Upon termination, the replisome is disassembled in two steps: first, CMG is ubiquitylated on its Mcm7 subunit by a cullin-RING E3 ubiquitin ligase (SCFDia2 in budding yeast, CUL2LRR1 in metazoa); second, ubiquitylated Mcm7 is unfolded by the Cdc48 ATPase (also known as p97 in higher eukaryotes), leading to disassembly of the replisome. Despite being driven by evolutionarily diverse E3 ubiquitin ligases in different eukaryotes (SCFDia2 in budding yeast, CUL2LRR1 in metazoa), replisome disassembly is governed by a common regulatory principle, in which ubiquitylation of CMG is suppressed before replication termination, to prevent replication fork collapse. Our structures show that the leucine-rich repeat domains of Dia2 and LRR1 are structurally distinct, but bind to a common site on CMG, including the MCM3 and MCM5 zinc-finger domains. The LRR–MCM interaction is essential for replisome disassembly and, crucially, is occluded by the excluded DNA strand at replication forks, establishing the structural basis for the suppression of CMG ubiquitylation before termination.

Nonetheless, we identified a subset of particles, which was subsequently subclassified into two conformations (conformations I and II), that had unambiguously translocated onto dsDNA, representative of bona fide termination intermediates produced after fork convergence. While the configuration of the MCM C-tier differed between conformations I and II, in both cases the incoming dsDNA was bent by approximately 46° between the MCM N-tier and C-tier, necessitating distortion of the DNA duplex within the N-tier. Having identified particles that had translocated onto dsDNA, we were able to build an atomic model of a terminated replisome. We observed an additional, large region of density at the N-tier face of CMG beside Mcm3 and Mcm7, which closely approaches Csm3 and the dsDNA ahead of CMG, before extending away from the core of the complex, forming an elongated arm characteristic of the cullin subunit (Cdc53) of SCFDia2. Density corresponding to the E3 ligase substrate-recognition module (Skp1–Dia2) is adjacent to the N-tier face of CMG. However, clearsecondary structure and side chain density enabled us to build a de novo atomic model for the remainder of Dia2, encompassing the F-box (residues 211–247), 15 tandem leucine-rich repeats (LRRs) (248–716) and a C-terminal tail (717–732), which folds back onto the concave surface of the horseshoe-shaped LRRs. The C-terminal end of the LRR domain forms an extensive interface with the N-tier of the Mcm3, Mcm5 and Mcm7 subunits of CMG (see text below for a detailed description), demonstrating that Dia2 binds directly to CMG bound around dsDNA, equivalent to the situation after convergence of two replication forks. The extensive interface between Dia2LRR and MCM is predominantly formed by the Mcm3 N-tier (helices α1 and α5 and the zinc-finger (ZnF) domain), which forms a cradle for the C terminus of Dia2LRR.

> MSDNRRRRREEDDSDSENELPPSSPQQHFRGGMNPVSSPIGSPDMINPEGDDNEVDDVPDIDEVEEQMNEVDLMDDNMYEDYAADHNRDRYDPDQVDDREQQELSLSERRRIDAQLNERDRLLRNVAYIDDEDEEQEGAAQLDEMGLPVQRRRRRRQYEDLENSDDDLLSDMDIDPLREELTLESLSNVKANSYSEWITQPNVSRTIARELKSFLLEYTDETGRSVYGARIRTLGEMNSESLEVNYRHLAESKAILALFLAKCPEEMLKIFDLVAMEATELHYPDYARIHSEIHVRISDFPTIYSLRELRESNLSSLVRVTGVVTRRTGVFPQLKYVKFNCLKCGSILGPFFQDSNEEIRISFCTNCKSKGPFRVNGEKTVYRNYQRVTLQEAPGTVPPGRLPRHREVILLADLVDVSKPGEEVEVTGIYKNNYDGNLNAKNGFPVFATIIEANSIKRREGNTANEGEEGLDVFSWTEEEEREFRKISRDRGIIDKIISSMAPSIYGHRDIKTAVACSLFGGVPKNVNGKHSIRGDINVLLLGDPGTAKSQILKYVEKTAHRAVFATGQGASAVGLTASVRKDPITKEWTLEGGALVLADKGVCLIDEFDKMNDQDRTSIHEAMEQQSISISKAGIVTTLQARCSIIAAANPNGGRYNSTLPLAQNVSLTEPILSRFDILCVVRDLVDEEADERLATFVVDSHVRSHPENDEDREGEELKNNGESAIEQGEDEINEQLNARQRRLQRQRKKEEEISPIPQELLMKYIHYARTKIYPKLHQMDMDKVSRVYADLRRESISTGSFPITVRHLESILRIAESFAKMRLSEFVSSYDLDRAIKVVVDSFVDAQKVSVRRQLRRSFAIYTLGH;> MKRRWKKNFIAVSAANRFKKISSSGALENLYFQGEAPVMEGSTGFDGDATTFFAPDAVFGDRVRRFQEFLDTFTSYRDSVRSIQVYNSNNAANYNDDQDDADERDLLGDDDGDDLEKEKKAASSTSLNILPHRIIISLDDLREFDRSFWSGILVEPAYFIPPAEKALTDLADSMDDVPHPNASAVSSRHPWKLSFKGSFGAHALSPRTLTAQHLNKLVSVEGIVTKTSLVRPKLIRSVHYAAKTGRFHYRDYTDATTTLTTRIPTPAIYPTEDTEGNKLTTEYGYSTFIDHQRITVQEMPEMAPAGQLPRSIDVILDDDLVDKTKPGDRVNVVGVFKSLGAGGMNQSNSNTLIGFKTLILGNTVYPLHARSTGVAARQMLTDFDIRNINKLSKKKDIFDILSQSLAPSIYGHDHIKKAILLMLMGGVEKNLENGSHLRGDINILMVGDPSTAKSQLLRFVLNTASLAIATTGRGSSGVGLTAAVTTDRETGERRLEAGAMVLADRGVVCIDEFDKMTDVDRVAIHEVMEQQTVTIAKAGIHTTLNARCSVIAAANPVFGQYDVNRDPHQNIALPDSLLSRFDLLFVVTDDINEIRDRSISEHVLRTHRYLPPGYLEGEPVRERLNLSLAVGEDADINPEEHSNSGAGVENEGEDDEDHVFEKFNPLLQAGAKLAKNKGNYNGTEIPKLVTIPFLRKYVQYAKERVIPQLTQEAINVIVKNYTDLRNDDNTKKSPITARTLETLIRLATAHAKVRLSKTVNKVDAKVAANLLRFALLGEDIGNDIDEEESEYEEALSKRSPQKSPKKRQRVRQPASNSGSPIKSTPRRSTASSVNATPSSARRILRFQDDEQNAGEDDNDIMSPLPADEEAELQRRLQLGLRVSPRRREHLHAPEEGSSGPLTEVGTPRLPNVSSAGQDDEQQQSVISFDNVEPGTISTGRLSLISGIIARLMQTEIFEEESYPVASLFERINEELPEEEKFSAQEYLAGLKIMSDRNNLMVADDKVWRV;> MSQQSSSPTKEDNNSSSPVVPNPDSVPPQLSSPALFYSSSSSQGDIYGRNNSQNLSQGEGNIRAAIGSSPLNFPSSSQRQNSDVFQSQGRQGRIRSSASASGRSRYHSDLRSDRALPTSSSSLGRNGQNRVHMRRNDIHTSDLSSPRRIVDFDTRSGVNTLDTSSSSAPPSEASEPLRIIWGTNVSIQECTTNFRNFLMSFKYKFRKILDEREEFINNTTDEELYYIKQLNEMRELGTSNLNLDARNLLAYKQTEDLYHQLLNYPQEVISIMDQTIKDCMVSLIVDNNLDYDLDEIETKFYKVRPYNVGSCKGMRELNPNDIDKLINLKGLVLRSTPVIPDMKVAFFKCNVCDHTMAVEIDRGVIQEPARCERIDCNEPNSMSLIHNRCSFADKQVIKLQETPDFVPDGQTPHSISLCVYDELVDSCRAGDRIEVTGTFRSIPIRANSRQRVLKSLYKTYVDVVHVKKVSDKRLDVDTSTIEQELMQNKVDHNEVEEVRQITDQDLAKIREVAAREDLYSLLARSIAPSIYELEDVKKGILLQLFGGTNKTFTKGGRYRGDINILLCGDPSTSKSQILQYVHKITPRGVYTSGKGSSAVGLTAYITRDVDTKQLVLESGALVLSDGGVCCIDEFDKMSDSTRSVLHEVMEQQTISIAKAGIITTLNARSSILASANPIGSRYNPNLPVTENIDLPPPLLSRFDLVYLVLDKVDEKNDRELAKHLTNLYLEDKPEHISQDDVLPVEFLTMYISYAKEHIHPIITEAAKTELVRAYVGMRKMGDDSRSDEKRITATTRQLESMIRLAEAHAKMKLKNVVELEDVQEAVRLIRSAIKDYATDPKTGKIDMNLVQTGKSVIQRKLQEDLSREIMNVLKDQASDSMSFNELIKQINEHSQDRVESSDIQEALSRLQQEDKVIVLGEGVRRSVRLNNRV;> MSFDRPEIYSAPVLQGESPNDDDNTEIIKSFKNFILEFRLDSQFIYRDQLRNNILVKNYSLTVNMEHLIGYNEDIYKKLSDEPSDIIPLFETAITQVAKRISILSRAQSANNNDKDPENTSMDTDSLLLNSLPTFQLILNSNANQIPLRDLDSEHVSKIVRLSGIIISTSVLSSRATYLSIMCRNCRHTTSITINNFNSITGNTVSLPRSCLSTIESESSMANESNIGDESTKKNCGPDPYIIIHESSKFIDQQFLKLQEIPELVPVGEMPRNLTMTCDRYLTNKVIPGTRVTIVGIYSIYNSKNGAGSGRSGGGNGGSGVAIRTPYIKILGIQSDVETSSIWNSVTMFTEEEEEEFLQLSRNPKLYEILTNSIAPSIFGNEDIKKAIVCLLMGGSKKILPDGMRLRGDINVLLLGDPGTAKSQLLKFVEKVSPIAVYTSGKGSSAAGLTASVQRDPMTREFYLEGGAMVLADGGVVCIDEFDKMRDEDRVAIHEAMEQQTISIAKAGITTVLNSRTSVLAAANPIYGRYDDLKSPGDNIDFQTTILSRFDMIFIVKDDHNEERDISIANHVINIHTGNANAMQNQQEENGSEISIEKMKRYITYCRLKCAPRLSPQAAEKLSSNFVTIRKQLLINELESTERSSIPITIRQLEAIIRITESLAKLELSPIAQERHVDEAIRLFQASTMDAASQDPIGGLNQASGTSLSEIRRFEQELKRRLPIGWSTSYQTLRREFVDTHRFSQLALDKALYALEKHETIQLRHQGQNIYRSGV;> MSSPFPADTPSSNRPSNSSPPPSSIGAGFGSSSGLDSQIGSRLHFPSSSQPHVSNSQTGPFVNDSTQFSSQRLQTDGSATNDMEGNEPARSFKSRALNHVKKVDDVTGEKVREAFEQFLEDFSVQSTDTGEVEKVYRAQIEFMKIYDLNTIYIDYQHLSMRENGALAMAISEQYYRFLPFLQKGLRRVVRKYAPELLNTSDSLKRSEGDEGQADEDEQQDDDMNGSSLPRDSGSSAAPGNGTSAMATRSITTSTSPEQTERVFQISFFNLPTVHRIRDIRSEKIGSLLSISGTVTRTSEVRPELYKASFTCDMCRAIVDNVEQSFKYTEPTFCPNPSCENRAFWTLNVTRSRFLDWQKVRIQENANEIPTGSMPRTLDVILRGDSVERAKPGDRCKFTGVEIVVPDVTQLGLPGVKPSSTLDTRGISKTTEGLNSGVTGLRSLGVRDLTYKISFLACHVISIGSNIGASSPDANSNNRETELQMAANLQANNVYQDNERDQEVFLNSLSSDEINELKEMVKDEHIYDKLVRSIAPAVFGHEAVKKGILLQMLGGVHKSTVEGIKLRGDINICVVGDPSTSKSQFLKYVVGFAPRSVYTSGKASSAAGLTAAVVRDEEGGDYTIEAGALMLADNGICCIDEFDKMDISDQVAIHEAMEQQTISIAKAGIHATLNARTSILAAANPVGGRYNRKLSLRGNLNMTAPIMSRFDLFFVILDDCNEKIDTELASHIVDLHMKRDEAIEPPFSAEQLRRYIKYARTFKPILTKEARSYLVEKYKELRKDDAQGFSRSSYRITVRQLESMIRLSEAIARANCVDEITPSFIAEAYDLLRQSIIRVDVDDVEMDEEFDNIESQSHAASGNNDDNDDGTGSGVITSEPPADIEEGQSEATARPGTSEKKKTTVTYDKYVSMMNMIVRKIAEVDREGAEELTAVDIVDWYLLQKENDLGSLAEYWEERRLAFKVIKRLVKDRILMEIHGTRHNLRDLENEENENNKTVYVIHPNCEVLDQLEPQDSS;> MSAALPSIQLPVDYNNLFNEITDFLVTFKQDTLSSDATRNENEDENLDAENIEQHLLEKGPKYMAMLQKVANRELNSVIIDLDDILQYQNEKFLQGTQADDLVSAIQQNANHFTELFCRAIDNNMPLPTKEIDYKDDVLDVILNQRRLRNERMLSDRTNEIRSENLMDTTMDPPSSMNDALREVVEDETELFPPNLTRRYFLYFKPLSQNCARRYRKKAISSKPLSVRQIKGDFLGQLITVRGIITRVSDVKPAVEVIAYTCDQCGYEVFQEVNSRTFTPLSECTSEECSQNQTKGQLFMSTRASKFSAFQECKIQELSQQVPVGHIPRSLNIHVNGTLVRSLSPGDIVDVTGIFLPAPYTGFKALKAGLLTETYLEAQFVRQHKKKFASFSLTSDVEERVMELITSGDVYNRLAKSIAPEIYGNLDVKKALLLLLVGGVDKRVGDGMKIRGDINVCLMGDPGVAKSQLLKAICKISPRGVYTTGKGSSGVGLTAAVMKDPVTDEMILEGGALVLADNGICCIDEFDKMDESDRTAIHEVMEQQTISISKAGINTTLNARTSILAAANPLYGRYNPRLSPLDNINLPAALLSRFDILFLMLDIPSRDDDEKLAEHVTYVHMHNKQPDLDFTPVEPSKMREYIAYAKTKRPVMSEAVNDYVVQAYIRLRQDSKREMDSKFSFGQATPRTLLGIIRLSQALAKLRLADMVDIDDVEEALRLVRVSKESLYQETNKSKEDESPTTKIFTIIKKMLQETGKNTLSYENIVKTVRLRGFTMLQLSNCIQEYSYLNVWHLINEGNTLKFVDDGTMDTDQEDSLVSTPKLAPQTTASANVSAQDSDIDLQDA;> MYGDLGNKLVLEAKRTKQLYARSNQDVNLPMYHEDIIRNILKEVSNLRKNTEYLKEQQQLGMLDDKVAKCQYFVTLLCMERNKRCLLAYQRLRTDILDSMAWNNNGLDLMSSITFSQQDTNNLSHQEQEYLKEYCDLITDLKSGDLVDIDLSGSLVPPSDVFIDVRVLKDAGEIQTEYGVFNLIKDSQFFVRQSDVERLIQQGYLQKI;> MSLPAHLQQTFSPEEIQFIVENEPIKIFPRITTRQKIRGDDRGTGNHTRWQLITTDDKALNNMVAMRSTEVVLWIALLLKQQSKCSIVAPQWLTTKELDRKIQYEKTHPDRFSELPWNWLVLARILFNKAKDDFHDPIHELRGKIQDLREIRQIKVLKGLKYLNESHLQLDNLSLLEINELRPFITEIMDKLREIHTASLTAGTENDEEEFNI;> MGYYDIDDVLADGTEFPCKFQYDIPGLGYLENNPGRPITKNTKLNLPLWLARILAIVGGDEALVDEEPVPFVELLPPDMFSTKVMNAIKTDPVALDLHSINSHFFSLAIKWIMLFSEKELANVVSELLLQRAQELNHHASSLSIDLNADSTGKNSANTNIATSTFLLKLEEMEKEIYKKSHESYKDTKRWMFKK;> MDINIDDILAELDKETTAVDSTKITQGSSSTTHRDANTIVGSSLDLNDKTQIYVSPQQDFSDLMKSWKNERCSPELLPYPHQLMKRLLNRISMQSQLIENISMGFLDMQNASNANPPMPNESKLPLLCMETELERLKFVIRSYIRCRLSKIDKFSLYLRQLNEDENSLISLTDLLSKDEIKYHDTHSLIWLKLVNDSILKYMPEELQAINDTEGSVNMIDEPDWNKFVFIHVNGPPDGKWNEDPLLQENEFGKPCYTVTIPDLKEEVELTIGSIYVMRYEVIRDLLRDDKVALI;> MYYGISQFSEAYNKILRNSSSHSSCQLVIFVSCLNIDALCATKMLSLLFKKQLVQSQIVPIFGYSELRRHYSQLDDNINSLLLVGFGGVIDLEAFLEIDPQEYVIDTDEKSGEQSFRRDIYVLDAHRPWNLDNIFGSQIIQCFDDGTVDDTLGEQKEAYYKLLELDEESGDDELSGDENDNNGGDDEATDADEVTDEDYKDDDGDYKDDDETISNKRGNSSIGPNDLSKRKQRKKQIHEYEGVLEEYYSQGTTVVNSISAQIYSLLSAIGETNLSNLWLNILGTTSLDIAYAQVYNRLYPLLQDEVKRLTPSSRNSVKTPDTLTLNIQPDYYLFLLRHSSLYDSFYYSNYVNAKLSLWNENGKKRLHKMFARMGIPLSTAQETWLYMDHSIKRELGIIFDKNLDRYGLQDIIRDGFVRTLGYRGSISASEFVEALTALLEVGNSTDKDSVKINNDNNDDTDGEEEEDNSAQKLTNLRKRWVSNFWLSWDALDDRKVELLNRGIQLAQDLQRAIFNTGVAILEKKLIKHLRIYRLCVLQDGPDLDLYRNPLTLLRLGNWLIECCAESEDKQLLPMVLASIDENTDTYLVAGLTPRYPRGLDTIHTKKPILNNFSMAFQQITAETDAKVRIDNFESSIIEIRREDLSPFLEKLTLSGLL;>[3x]MKRRWKKNFIAVSAANRFKKISSSGALENLYFQGEMVSVIDKLVFDFGGKTLVSLAPDNNTLCVANKNGLTKILKTNNPEEEPETLDSSKLVSSIKCYSNSHFLMTTMQGDALRYNIDSSQEELLARFALPLRDCCVIHSGKMAVFGGDDLELILLELDDETHKKHAIKIDEQVSQISYNSQMNILAVSMINGKVQIFSLTSTIPNKVHELNDYIVANSYDDTHRDKILSNMMDDIDKDNDNDLSETADPDENNVADPEFCAANRICTRVAWHPKGLHFALPCADDTVKIFSIKGYSLQKTLSTNLSSTKAHFIDLQFDPLRGTYIAAVDLNNKLTVWNWETSEIHYTREFKRKITNIAWKIQADSKTLDLVLGTWSGSIAIVQNLAESVVSNIPDQSVAESSTKHGLFVDSESDLENLEGNDDINKSDKLFSDITQEANAEDVFTQTHDGPSGLSEKRKYNFEDEEDFIDDDDGAGYISGKKPHNEHSYSRVHKTHSFPISLANTGKFRYMPFSPAGTPFGFTDRRYLTMNEVGYVSTVKNSEQYSITVSFFDVGRFREYHFEDLFGYDLCFLNEKGTLFGQSKTGQIQYRPHDSIHSNWTKIIPLQAGERITSVAATPVRVIVGTSLGYFRSFNQFGVPFAVEKTSPIVALTAQNYRVFSVHYSQFHGLSYSLSELGTSSKRYYKRECPLPMSLPNINSDMKKDANLDYYNFNPMGIKSLFFSSYGDPCIFGSDNTLLLLSKWRSPEESKWLPILDSNMEIWKMSGGKETTDIHVWPLALAYDTLNCILVKGKHIWPEFPLPLPSEMEIRMPVFVKSKLLEENKAILNKKNEIGADTEAEEGEEDKEIQIPVSMAAEEEYLRSKVLSELLTDTLENDGEMYGNENEVLAALNGAYDKALLRLFASACSDQNVEKALSLAHELKQDRALTAAVKISERAELPSLVKKINNIREARYEQQLK;> MVTSNVVLVSGEGERFTVDKKIAERSLLLKNYLNDMHDSNLQNNSDSESDSDSETNHKSKDNNNGDDDDEDDDEIVMPVPNVRSSVLQKVIEWAEHHRDSNFPDEDDDDSRKSAPVDSWDREFLKVDQEMLYEIILAANYLNIKPLLDAGCKVVAEMIRGRSPEEIRRTFNIVNDFTPEEEAAIRRENEWAEDR;> GAGMSSPGNSGVAIDSTVLKAIELGTRLFKSGEYLQAKRIFTNALRVCDSYSQEQIMRIRNAYQLDTARPDNKRLYHPRYIKILDNICACYEKLNDLKSCLDVSQRLLKLEPGNIKCYIRCTRTLIKLKDWKRAYKTCSRGLQLCNNDSNHLRQQKQFIKNNMVQKQDGKRSYIDPLEETKIAKKKKNNNVLESLPKKKIKGSTKKTDLVGNLPIEILPIIFQRFTTKELVTLSLVCNKWRDKILYHLDCFQEFNLAPINFKNFVKFMDFLQQNFTRTYRKYILSQVKVSSRITSEELRITQLLFSKMPKCINIERLILSMPTLTTTQIFKLMVRGGTDFFTRLLELSLMITYRPDKQHELEILQTCPLLKKIELIFVNSLVPIFDGNNSVGRDGSFNVMARHTNMQISTADNDEQGIVEEKVIYSELEKITLICDKKKIKNFPLCRALLRGQFPLLQKLTITGVTFPMNNQDIMNFQWLLNFPDLKELWIEDNDNCELSKFLQLLKFSNVWKNLEKLTFRENKLYPIVNLDEDQPVTNDDEVPSMLFYKENLQNLEKLDLMGTSISGSALTRLCEQEYLDGRKLRSLNIGNCPNIQFPNNHAHTARMILDVNAVLKRLSKLEEINLSHLSSLNDSTMKSFIINVPFLENLKRLDISHNFEITGISIYEFLKKFQMDHDNEAGGQPLAYLNIDGCSQVSHITVNMIRAQNLVTQVDCVYERDVWRKFGINSYSYS;> MMFGKKKNNGGSSTARYSAGNKYNTLSNNYALSAQQLLNASKIDDIDSMMGFERYVPPQYNGRFDAKDIDQIPGRVGWLTNMHATLVSQETLSSGSNGGGNSNDGERVTTNQGISGVDFYFLDEEGGSFKSTVVYDPYFFIACNDESRVNDVEELVKKYLESCLKSLQIIRKEDLTMDNHLLGLQKTLIKLSFVNSNQLFEARKLLRPILQDNANNNVQRNIYNVAANGSEKVDAKHLIEDIREYDVPYHVRVSIDKDIRVGKWYKVTQQGFIEDTRKIAFADPVVMAFAIATTKPPLKFPDSAVDQIMMISYMIDGEGFLITNREIISEDIEDFEYTPKPEYPGFFTIFNENDEVALLQRFFEHIRDVRPTVISTFNGDFFDWPFIHNRSKIHGLDMFDEIGFAPDAEGEYKSSYCSHMDCFRWVKRDSYLPQGSQGLKAVTQSKLGYNPIELDPELMTPYAFEKPQHLSEYSVSDAVATYYLYMKYVHPFIFSLCTIIPLNPDETLRKGTGTLCEMLLMVQAYQHNILLPNKHTDPIERFYDGHLLESETYVGGHVESLEAGVFRSDLKNEFKIDPSAIDELLQELPEALKFSVEVENKSSVDKVTNFEEIKNQITQKLLELKENNIRNELPLIYHVDVASMYPNIMTTNRLQPDSIKAERDCASCDFNRPGKTCARKLKWAWRGEFFPSKMDEYNMIKRALQNETFPNKNKFSKKKVLTFDELSYADQVIHIKKRLTEYSRKVYHRVKVSEIVEREAIVCQRENPFYVDTVKSFRDRRYEFKGLAKTWKGNLSKIDPSDKHARDEAKKMIVLYDSLQLAHKVILNSFYGYVMRKGSRWYSMEMAGITCLTGATIIQMARALVERVGRPLELDTDGIWCILPKSFPETYFFTLENGKKLYLSYPCSMLNYRVHQKFTNHQYQELKDPLNYIYETHSENTIFFEVDGPYKAMILPSSKEEGKGIKKRYAVFNEDGSLAELKGFELKRRGELQLIKNFQSDIFKVFLEGDTLEGCYSAVASVCNRWLDVLDSHGLMLEDEDLVSLICENRSMSKTLKEYEGQKSTSITTARRLGDFLGEDMVKDKGLQCKYIISSKPFNAPVTERAIPVAIFSADIPIKRSFLRRWTLDPSLEDLDIRTIIDWGYYRERLGSAIQKIITIPAALQGVSNPVPRVEHPDWLKRKIATKEDKFKQTSLTKFFSKTKNVPTMGKIKDIEDLFEPTVEEDNAKIKIARTTKKKAVSKRKRNQLTNEEDPLVLPSEIPSMDEDYVGWLNYQKIKWKIQARDRKRRDQLFGNTNSSRERSALGSMIRKQAESYANSTWEVLQYKDSGEPGVLEVFVTINGKVQNITFHIPKTIYMKFKSQTMPLQKIKNCLIEKSSASLPNNPKTSNPAGGQLFKITLPESVFLEEKENCTSIFNDENVLGVFEGTITPHQRAIMDLGASVTFRSKAMGALGKGIQQGFEMKDLSMAENERYLSGFSMDIGYLLHFPTSIGYEFFSLFKSWGDTITILVLKPSNQAQEINASSLGQIYKQMFEKKKGKIETYSYLVDIKEDINFEFVYFTDISKLYRRLSQETTKLKEERGLQFLLLLQSPFITKLLGTIRLLNQMPIVKLSLNEVLLPQLNWQPTLLKKLVNHVLSSGSWISHLIKLSQYSNIPICNLRLDSMDYIIDVLYARKLKKENIVLWWNEKAPLPDHGGIQNDFDLNTSWIMNDSEFPKINNSGVYDNVVLDVGVDNLTVNTILTSALINDAEGSDLVNNNMGIDDKDAVINSPSEFVHDAFSNDALNVLRGMLKEWWDEALKENSTADLLVNSLASWVQNPNAKLFDGLLRYHVHNLTKKALLQLVNEFSALGSTIVYADRNQILIKTNKYSPENCYAYSQYMMKAVRTNPMFSYLDLNIKRYWDLLIWMDKFNFSGLACIEIEEKENQDYTAVSQWQLKKFLSPIYQPEFEDWMMIILDSMLKTKQSYLKLNSGTQRPTQIVNVKKQDKEDSVENSLNGFSHLFSKPLMKRVKKLFKNQQEFILDPQYEADYVIPVLPGSHLNVKNPLLELVKSLCHVMLLSKSTILEIRTLRKELLKIFELREFAKVAEFKDPSLSLVVPDFLCEYCFFISDIDFCKAAPESIFSCVRCHKAFNQVLLQEHLIQKLRSDIESYLIQDLRCSRCHKVKRDYMSAHCPCAGAWEGTLPRESIVQKLNVFKQVAKYYGFDILLSCIADLTI;> MFGSGNVLPVKIQPPLLRPLAYRVLSRKYGLSIKSDGLSALAEFVGTNIGANWRQGPATIKFLEQFAAVWKQQERGLFIDQSGVKEVIQEMKEREKVEWSHEHPIQHEENILGRTDDDENNSDDEMPIAADSSLQNVSLSSPMRQPTERDEYKQPFKPESSKALDWRDYFKVINASQQQRFSYNPHKMQFIFVPNKKQNGLGGIAGFLPDIEDKVQMFLTRYYLTNDRVMRNENFQNSDMFNPLSSMVSLQNELSNTNRQQQSSSMSITPIKNLLGRDAQNFLLLGLLNKNFKGNWSLEDPSGSVEIDISQTIPTQGHYYVPGCMVLVEGIYYSVGNKFHVTSMTLPPGERREITLETIGNLDLLGIHGISNNNFIARLDKDLKIRLHLLEKELTDHKFVILGANLFLDDLKIMTALSKILQKLNDDPPTLLIWQGSFTSVPVFASMSSRNISSSTQFKNNFDALATLLSRFDNLTENTTMIFIPGPNDLWGSMVSLGASGTLPQDPIPSAFTKKINKVCKNVVWSSNPTRIAYLSQEIVIFRDDLSGRFKRHRLEFPFNESEDVYTENDNMMSKDTDIVPIDELVKEPDQLPQKVQETRKLVKTILDQGHLSPFLDSLRPISWDLDHTLTLCPIPSTMVLCDTTSAQFDLTYNGCKVINPGSFIHNRRARYMEYVPSSKKTIQEEIYI;> MSADLQQGTTNAADFSLTVLRARIALLATAIGGPDYTSQIDPPPYKLGDDCLACLKDLKRWFKLVDDQQKRWDVAMAVAEYRILTDDLLPILIDWENKCSLAAKLAKNNPDHEEFRNKAYYDKIALNCLQLLVLMTWPLIVTEQSSSNQITLYGELKKHQLVYKKTILSMESGKVLRAAIRLALDVIKIDRLSRTPRDNMVLKLVLNFFRNVIAIEPGEFTINTKKSMPKKGITSIDTLPPNVSMDDISLNTVISSFHKNKVFGFLLTLTSSLSKEFDQDFINIPLLEIMFYFTKDVNQELLFPRQFETGTHSKVVNKNESSSANNIVTSAGFELSKLLQKEHQMRKNVIKHTSARHSRFGGLLSIQTPDKTRLTVSGSQALVDEKIALQKLDDSKKWNKRIIKKHQSVAAEGLPNSLLNSQTGKAIFFTESNGKHFKEFINNFIDSGFNILLHSVTNYFTTEQDRMVTLEQVEYLLFFAWFVKYQLLRSKIDNSADIKQVSEALKEVTFILVSSLLRSAYDLKNWTVTHAGMIAFNELLNLVSRTKAAQEEDSTDIEFIVSRLFSDERIQLLSNLPKIGSKYSLQFMKSCIELTHSVLKVLEQYSDDKTLVIEGKSRRQKKFNISEGDITKLIEEENVDRDEALDILTSSLRSIEVNFQKVQANYMTEPVIETYINFLERFRELEDDSIKKVFSFFHRVFVQAKEQALLFRFDLIILLREMLSPDGLDRMSRSRKYVSQFSDYFLARLKKRLKKSPAWFVGLLFPPLHNSEVGFYQRYGEYNVLNNESMYAAPASQFKPIPDEEALPPSILLDMKYGVLVSTLLDDGKTELLDQLLKHITHTLDIFKSWLTVNVNAGKETVNPPNEYFTLTGVLNNDPIFKDKDYRALLLLIGYSIPRKINEPCFLPGTVEVSDLTVSCELVKKYLSTPFETPNGLPSSSYLLRVRSEKDSFSHNEQDGWEGDDDYDYNDPYIVPDDQILSKSDAAYFKDLDNNASDKLKGTKFSKGIARSKKKDKRKRRKGEAKTNLPMFGDQDDERPQTVRERHGVFSKEFISDSEDDEDLMNPIFFENETYMRWLLDKNNGQLTEDRYIQFAKFAAERMNNGGVVTGDYTSLFGGSIPSIESIRATESSSFAPDKSLISLASHVASEMSIFDVNNNNNNQLSDDDVNSESRNSLGSSQPSNSQNMFQSEVYSRKESTKRSLEASAADESDEDEEAIRLFGKKSRVVLSQGDSDD;> GEMDQDFDSLLLGFNDSDSVQKDPTVPNGLDGSVVDPTIADPTAITARKRRPQVKLTAEKLLSDKGLPYVLKNAHKRIRISSKKNSYDNLSNIIQFYQLWAHELFPKAKFKDFMKICQTVGKTDPVLREYRVSLFRDEMGMSFDVGTRETGQDLERQSPMVEEHVTSAEERPIVADSFAQDKRNVNNVDYDNDEDDDIYHLSYRNRRGRVLDERGNNETVLNNVVPPKEDLDALLKTFRVQGPVGLEENEKKLLLGWLDAHRKMEKGSMTEEDVQLIQSLEEWEMNDIEGQHTHYDLLPGGDEFGVDQDELDAMKEMGF> MATQQPALVLDPTGADHHTEHRTLREGGPATWVDVLGVQAWSVSDPVLLKQLLTSSDVSKDARAHWPAFGEVVGTWPLALWVAVENMFTAYGPNHRKLRRLVAPAFSARRVDAMRPAVEAMVTGLVDRLAELPAGEPVDLRQELAYPLPIAVIGHLMGVPQDRRDGFRALVDGVFDTTLDQAE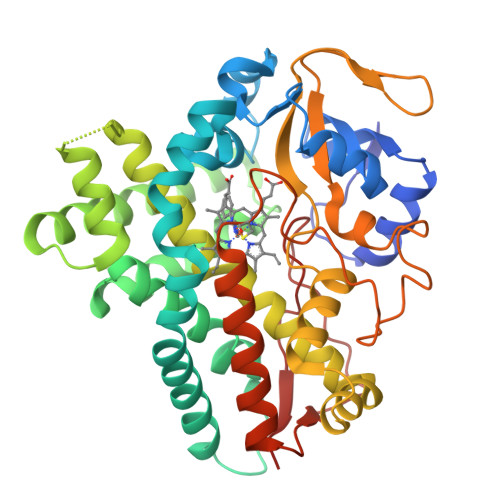AQANTARLYEVLDQLIAAKRATPGDDMTSLLIAARDDEGDGDRLSPEELRDTLLLMISAGYETTVNVIDQAVHTLLTRPDQLALVRKGEVTWADVVEETLRHEPAVKHLPLRYAVTDIALPDGRTIARGEPILASYAAANRHPDWHEDADTFDATRTVKEHLAFGHGVHFCLGAPLARMEVTLALESLFGRFPDLRLADPAEELPPVPSLISNGHQRLPVLLHAG> PISPIETVPVKLKPGMDGPKVKQWPLTEEKIKALVEICTEMEKEGKISKIGPENPYNTPVFAIKKKDSTKWRKLVDFRELNKRTQDFWEVQLGIPHPAGLKKKKSVTVLDVGDAYFSVPLDEDFRKYTAFTIPSINNETPGIRYQYNVLPQGWKGSPAIFQSSMTKI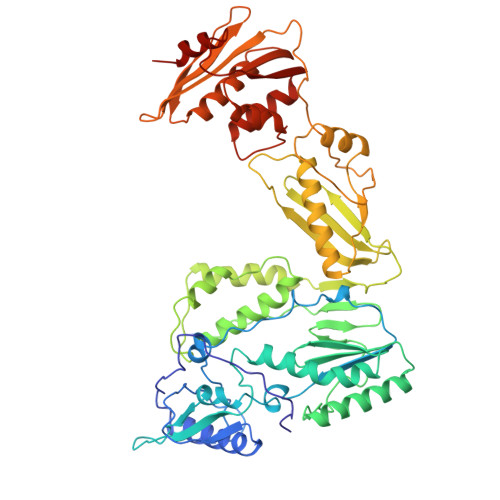LEPFKKQNPDIVIYQYMDDLYVGSDLEIGQHRTKIEELRQHLLRWGLTTPDKKHQKEPPFLWMGYELHPDKWTVQPIVLPEKDSWTVNDIQKLVGKLNWASQIYPGIKVRQLCKLLRGTKALTEVIPLTEEAELELAENREILKEPVHGVYYDPSKDLIAEIQKQGQGQWTYQIYQEPFKNLKTGKYARMRGAHTNDVKQLTEAVQKITTESIVIWGKTPKFKLPIQKETWETWWTEYWQATWIPEWEFVNTPPLVKLWYQLEKEPIVGAETFYVDGAANRETKLGKAGYVTNKGRQKVVPLTNTTNQKTELQAIYLALQDSGLEVNIVTDSQYALGIIQAQPDKSESELVNQIIEQLIKKEKVYLAWVPAHKGIGGNEQVDKLVSA>[2x]YKWHYSGLNRWHGAGSTADFQKIIQERCDTYTQTIRPGSRSRNCQAIRQAFMSAFISKDPCKATKEDYNSLINLAPPTVPCGQQVFWSKTKELAHEYAKRRRLMTLED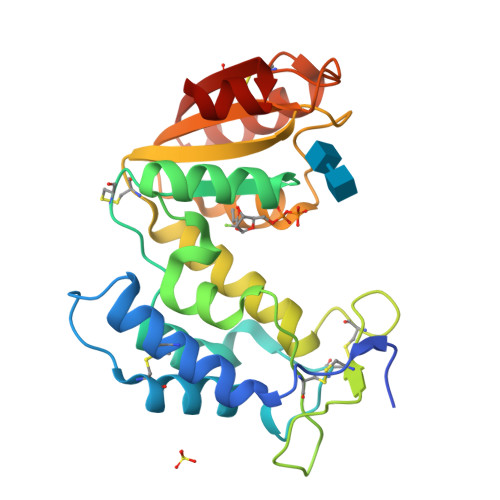TLLGYLADGLRWCGEPGSSDLNIWSCPDWRKDCRTNYLSVFWEVLSERFAESACNTVRVVLNGSLENAFDSMSIFGRVEAPNLRPQVELEAWLVHDTGKPPSDSCSGSSIRKLKSILDGRNVKFRCMDNLSRDQFLQRS methyl 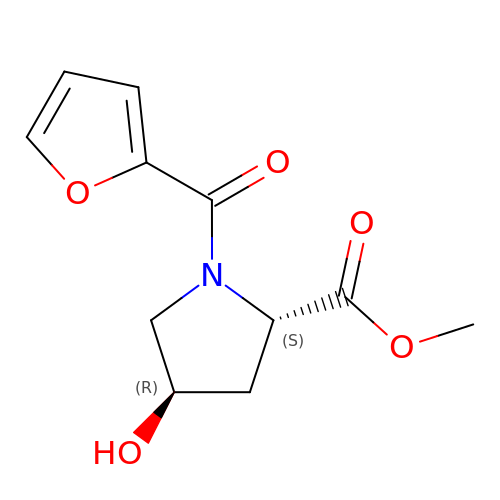(2~{S},4~{R})-1-(furan-2-ylcarbonyl)-4-oxidanyl-pyrrolidine-2-carboxylate | C11 H13 N O5 | GVYWVRYDCMRUCE-SFYZADRCSA-N> GGCCGUUCGGGCGGCCAUAAACAGCCCUCAGACCCGAAGCGUGGCGUUCC;> GGAACGCCGGUG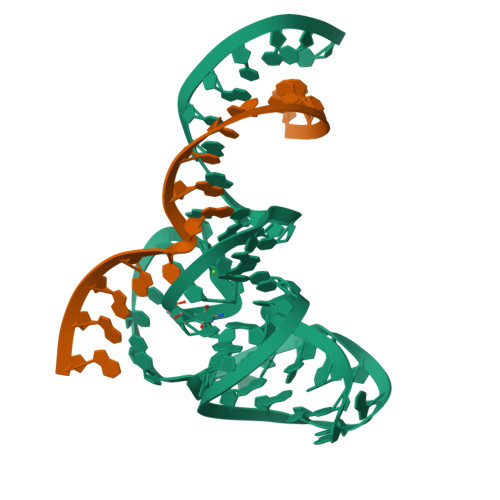GGA>SMKQYRNFVDGKWVESSKTFQDVTPIDGSVVAVVHEADRDLVDAAVKAGHRALEGEWGRTTAAQRVDWLRRIANEMERRQQDFLDAEMADTGKPLSMAATIDIPRGIANFRNFADILATAPVDSHRLDLPDGAYALNYAARKPLGVVGVISPWNLPLLLLTWKVAPALACGNAVVVKPSEDTPGTATLLAEVMEAVGIPPGVFNLVHGFGPNSAGEFISQHPDISAITFTGESKTGSTIMRAAAEGVKPVSFELGGKNAAVIFADCDFEKMLDGMMRALFLNSGQVCLCSERVYVERPIFDRFCVALAERIKALKVDWPHETDTQMGPLISSKHRDKVLSYFELARQEGATFLAGGGVPRFGDERDNGAWVEPTVIAGLSDDARVVREEIFGPICHVTPFDSESEVIRRANDTRYGLAATIWTTNLSRAHRVSELMRVGISWVNTWFLRDLRTPFGGAGLSGIGREGGMHSLNFYSE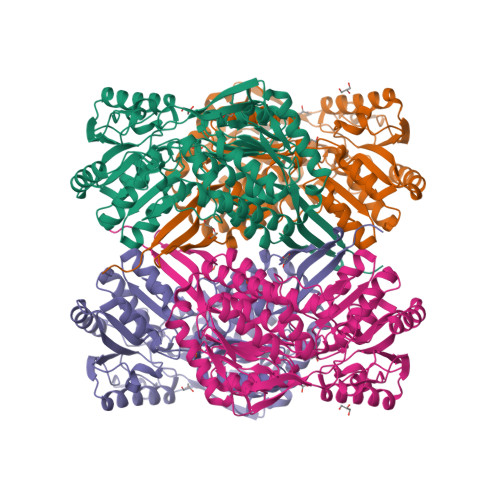LTNVCVRIDKESPDV[2x]> MEFTVSTTEDLQRYRTECVSSLNIPADYVEKFKKWEFPEDDTTMCYIKCVFNKMQLFDDTEGPLVDNLVHQLAHGRDAEEVRTEVLKCVDKNTDNNACHWAFRGFKCFQKNNLSLIKASIKKD

Ae. aegypti OBP22 (AeOBP22) is a member of the OBP family of proteins that has been directly implicated in regulating these feeding behaviors. AeOBP22 is unusual in that it is expressed in multiple chemosensory tissues, including in the antenna, the proboscis of the females, the thoracic spiracles, in the male reproductive glands where it is transferred to the females during mating, and in the salivary glands. The monomeric forms of AeOBP22 are similar to other classical OBPs which consist of six α-helices stabilized by three disulfide bridges surrounding a hydrophobic pocket. Our results provide evidence that fatty acids are likely natural ligands for AeOBP22 and that the binding of long-chain fatty acids (C15-C20) is enhanced by a conformational change in the C-terminal tail that is critical to generate a high affinity binding site.

Other compounds can produce the same magnitude of NMR chemical shift changes, notably geraniol, citronellol and benzaldehyde. However, this only occurred at high ligand concentrations (typically> 1 mM) and binding is weak as exemplified by the concentration dependence of the chemical shift changes. Initial crystals formed in the P3121 space group, and the structure was solved using single wavelength anomalous dispersion (SAD) of a tantalum bromide (Ta6Br12) soaked crystal refined at 2.6 Å resolution. A native data set collected on the same crystal was refined at a resolution of 1.9 Å to an R/RFree of 18.3/20.1%. In this crystal form the protein forms a domain swapped dimer, with residues 116–122 of one molecule forming an anti-parallel β-sheet with residues 37–41 in a symmetry related molecule. For AeOBP22 the predicted molecular weights from multiple measurements of the R2/R1 ratios in both apo and fatty acid bound states were in the range 14.1–15.2 KDa, in agreement with the expected molecular weight of 14.3 KDa, indicating that the protein exists as monomers in the absence of other binding partners. We saw no evidence of any significant dimerization over long periods even at the high concentrations used for NMR chemical shift assignments (600–700 μM). Therefore, we conclude that the domain swapped dimers are an artifact of the crystallization process, and further discussions below are confined to the structures of the monomeric forms.>[2x]GPLGSGSGHLAIGSAATLGSGGMARGREPGGVGHVVAQVQSVDGNAQCCDCREPAPEWASINLGVTLCIQCSGIHRSLGVHFSK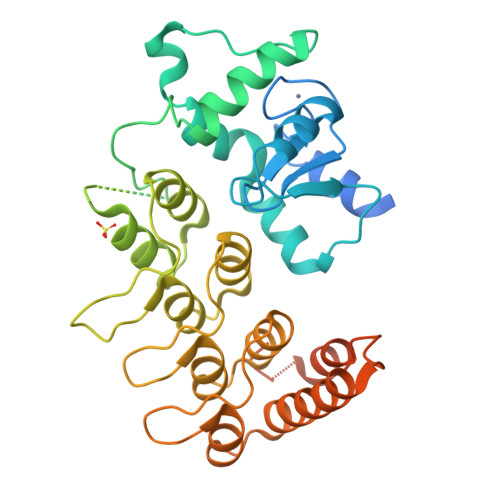VRSLTLDSWEPELVKLMCELGNVIINQIYEARVEAMAVKKPGPSCSRQEKEAWIHAKYVEKKFLTKLPEIRGRRGGRGRPRGQPPVPPKPSIRPRPGDLRSKPEPPSEDLGSLHPGALLFRASGHPPSLPTMADALAHGADVNWVNGGQDNATPLIQATAANSLLACEFLLQNGANVNQADSAGRGPLHHATILGHTGLACLFLKRGADLGARDSEGRDPLTIAMETANADIVTLLRLAKMREAEAAQGQAGDETYLDIFRDFSLMASDDPEKLSRRSHDLHTLGSSNSGSNSGHDRREFAKFEKE> GPGYQDPARSVRHIAIPAHRGLITDRNGEPLAVSTPVTTLWANPKELMTAKERWPQLAAALGQDTKLFADRIEQNAEREFIYLVRGLTPEQGEGVIALKVPGVYSIEEFRRFYPAGEVVAHAVGFTDVDDRGREGIELAFDEWLAGVPGKRQVLKDRRGRVIKDVQVTKNAKPGKTLALSIDLRLQYLAHRELRNALLENGAKAGSLVIMDVKTGEILAMTNQPTYNPNNRRNLQPAAMRNRAMIDVFEPGSTVKPFSMSAALASGRWKPSDIVDVYPGTLQ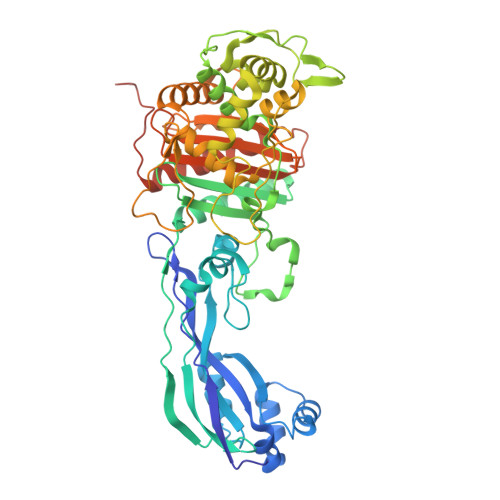IGRYTIRDVSRNSRQLDLTGILIKSSNVGISKIAFDIGAESIYSVMQQVGLGQDTGLGFPGERVGNLPNHRKWPKAETATLAYGYGLSVTAIQLAHAYAALANDGKSVPLSMTRVDRVPDGVQVISPEVASTVQGMLQQVVEAQGGVFRAQVPGYHAAGKSGTARKVSVGTKGYRENAYCSLFAGFAPATDPRIAMVVVIDEPSKAGYFGGLVSAPVFSKVMAGALRLMNVPPDNLPTATEQQQVNAAPAKGGRG(2E)-3-{5-[(2,4-diamino-6-propylpyrimidin-5-yl)methyl]-2,3-dimethoxyphenyl}-1-[(1S)-1-(2-methylprop-1-en-1-yl)phthalazin-2(1H)-yl]prop-2-en-1-one 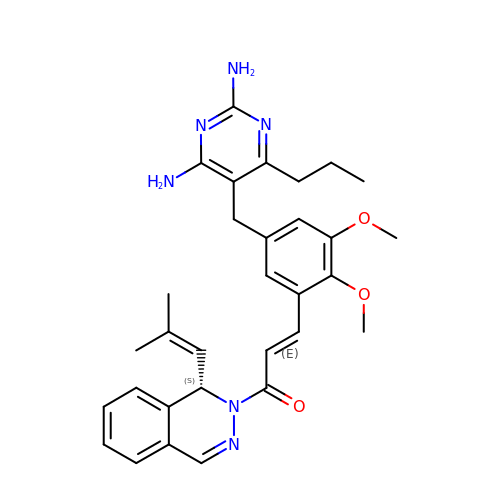| C31 H36 N6 O3 | FJDNNCPVIFOVAR-JYSHFMIGSA-N> MSEDIRRGPGRPPKKRVVPNFERKGILEKPVRPQSRLEFSYDNPLIFKNLFIYFKNLKSKNILVRCTPTEITFFSRDQSQA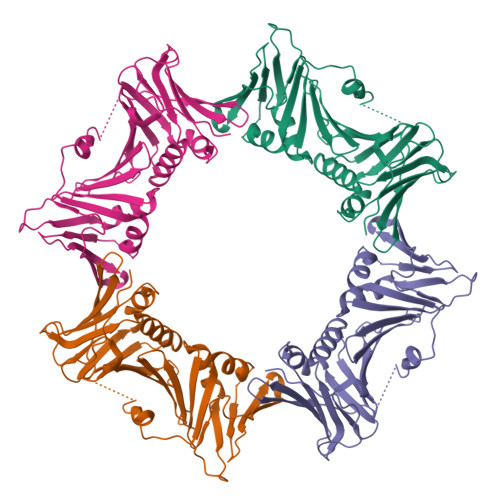SFVIATIDGKNVNHYYASDVFWLGINRELVEKMFNSIDRSFLKITIVHRYDKPETLFFIFTDFDIDKECTYQITVSEPELDMDLIEMEKSISEERLKNYPLRWEFTSKQLKKTFSDLSNYTELVTIEKLGGDTPLHLYFQKFNSISYHEMYKSSNKINLTSTIPKSQVFQINVKIAHIKSLASAMVTDKIRILCEENGNLIFQSEMDALMLNTITLNNTI>GGRMQLTADQVEKYKSDGYVLLEGAFSPEEVHVMRQALKKDQEVQGPHRILEEDGRTVRALYASHTRQSVFDQLSRSDRLLGPATQLLECDLYIHQFKINTKRAFGGDSWAWHQDFIVWRDTDGLPAPRAVNVGVFLSDVTEFNGPVVFLSGSHQRGTVERKARETSRSDQHVDPDDYSMTPAELSQMVEKHPMVSPKAASGSVMLFHPEIIHGSAPNISPFARDLLIITYNDVANAPKPAGEPRPEYVIGRDTTPLVSRSGPLHEAA[2x]

Like LdoA and EcdK, GriE belongs to the 2OG-Fe(ii) oxygenase superfamily, whose members couple the decarboxylation of α-ketoglutarate to substrate oxygenation/hydroxylation via an oxo-ferryl intermediate. Recombinant GriH purified from S. lividans TK24 lacked the characteristic fluorescence of the expected F420 co-factor but nevertheless led to 4-MePro in a coupled assay with GriF, indicating that GriH can use NADH directly without requiring F420. Together, these experiments suggest that 4-MePro biosynthesis starts with the GriE-mediated hydroxylation of l-leucine, followed by oxidation with GriF. The crystal structures of the leucine hydroxylase GriE have been determined in complex with substrates and products, providing insight into the stereospecificity of the reaction.

The canonical iron-binding motif is formed by His110, Asp112 and His210 and has lost the metal in the apo structure. The crystal structure obtained by co-crystallization with Co2+ and substrates unambiguously revealed bound metal and both l-leucine and α-ketoglutarate (Fig. S8A and B†). Co2+ is coordinated by the iron-binding motif and by α-ketoglutarate as a bi-dentate ligand through its C-1 carboxylate and C-2 keto group (6A and S9†). The axial position trans to His110, the expected binding site of oxygen, remains vacant. l-Leucine does not coordinate to the metal ion but is tightly bound via its carboxy and amino groups. Its side chain is not involved in the interactions and adopts a conformation that corresponds to the most probable rotamer (Fig. S10†). The coordination site trans to His110 remains vacant. This crystal structure should thus correspond to the substrate complex prior to the binding of dioxygen to the unoccupied coordination site of Fe(ii). In the GriE/substrate complex, both the Cδ methyl groups of l-leucine are located at a 4.4 Å distance to the metal. The reactive oxygen atom should be coordinated to the metal in a distance of approx. 1.6 Å.19–21 With respect to this position, the pro-S group would be closer to the reactive oxygen atom (3.0 Å) than the other Cδ methyl group (3.3 Å), explaining the exclusive formation of (2S,4R)-5-hydroxyleucine (Fig. 6A and S9†).> SHSTAETTLDSFFSRAGLVGEIDLPLEGTTNP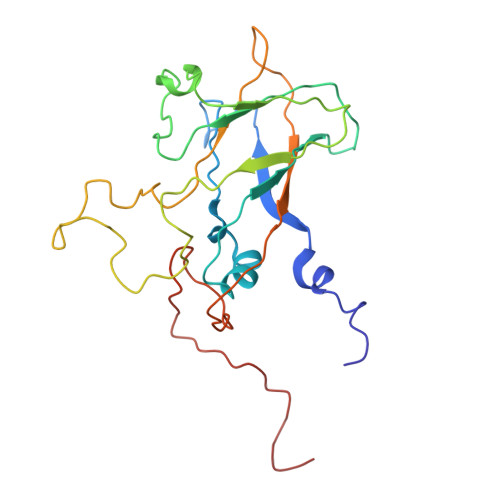NGYANWDIDITGYAQMRRKVELFTYMRFDAEFTFVACTPTGQVVPQLLQYMFVPPGAPKPDSRESLAWQTATNPSVFVKLSDPPAQVSVPFMSPASAYQWFYDGYPTFGEHKQEKDLEYGACPNNMMGTFSVRTVGTSKSKYPLVIRIYMRMKHVRAWIPRPMRNQNYLFKANPNYAGNFIKPTGASRTAITT>MHHHHHHHHGSENLYFQGSGEEVSEEGFQIPATITERYKVGRTIGDGNFAVVKECVERSTAREYALKIIKKSKCRGKEHMIQNEVSILRRVKHPNIVLLIEEMDVPTELYLVMELVKGGDLFDAITSTNKYTERDASGMLYNLASAIKYLHSLNIVHRDIKPENLLVYEHQDGSKSLKLGDFGLATIVDGPLYTVCGTPTYVAPEIIAETGYGLKVDIWAAGVITYILLCGFPPFRGSGDDQEVLFDQILMGQVDFPSPYWDNVSDS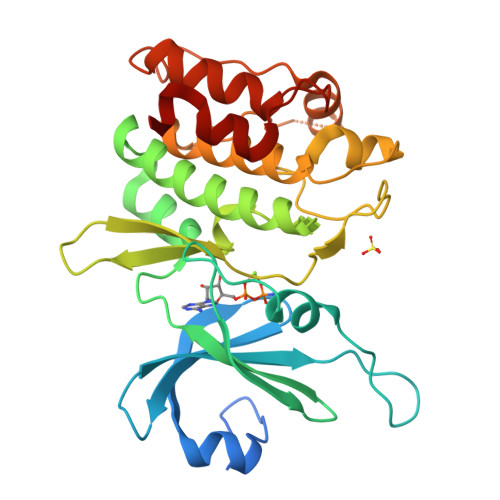AKELITMMLLVDVDQRFSAVQVLEHPWVND[2x]>AAKPKLYYFNGRGRMESIRWLLAAAGVEFEEEFLETREQYEKMQKDGHLLFGQVPLVEIDGMMLTQTRAILSYLAAKYNLYGKDLKERVRIDMYADGTQDLMMMIAVAPFKTPKEKEESYDLILSRAKTRYFPVFEKILKDHGEAFLVGNQLSWADIQLLEAILMVEELSAPVLSDFPLLQAFKTRISNIPTIKKFLQPGSQRKPPP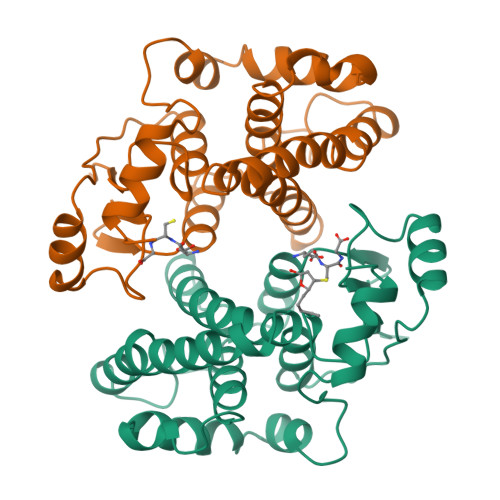DGPYVEVVRIVLKF[2x]>[4x]MNDNVAWFKQAKYGMMIHWGLYSLLAGEYRGESSSAYAEWIQSKFQIPNAEYGNLATAFNPLYFDAK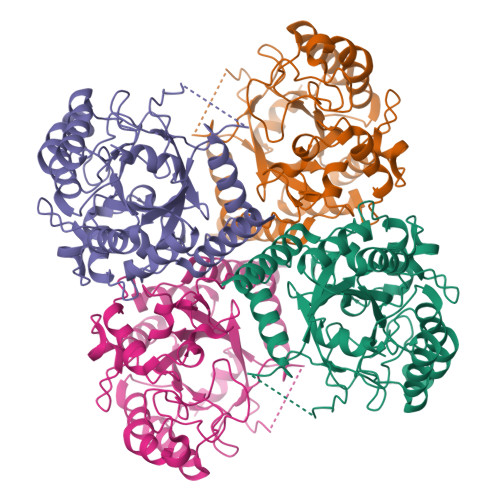KIVALAKQCGMQYLVVTTKHHDGFAMYHSKVDAYNVYDATPFHRDIIGELAEACQKAGLKFGLYYSQDLDWHDPNGGGYKSNDVETAGTTWDNSWDFPDEDQKNFDLCFDNKILPQIKEIMSNYGDIATAWFDVPMTLSEAQSQTIYDTVRELQPNCLINSRLGNGKYDFVSLGDNEIPKNKEDMNKTDVDYNEITGFKPSPLGLYATAGTINDSWGFSYHDQNWKTPRTLYRYKQHLNDFGINYLLNVGLDPLGRVPMMAEENLLAAKALEDEANRL>GXCCCGGG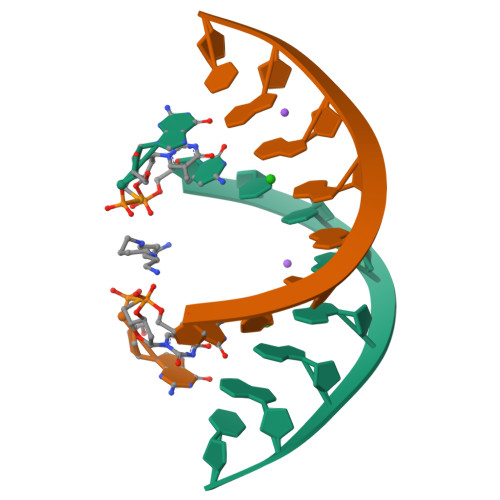AC[2x]> ASMTIVDCGPPDDLPSGRVEYITGPGVTTYKAVIQYSCEETFYTMKVNDGKYVC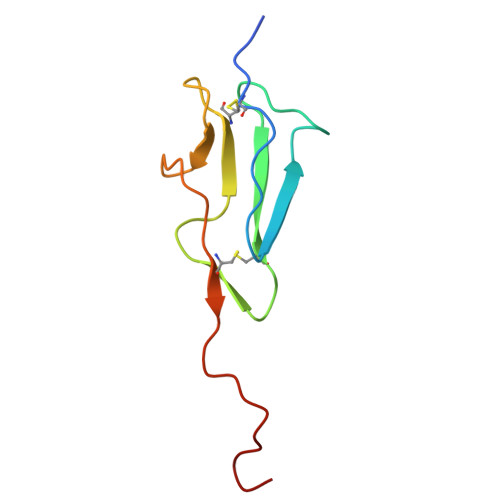DADGFWTSSKGEKSLPVCEPVCGLSARTTGGR> GGTGGGG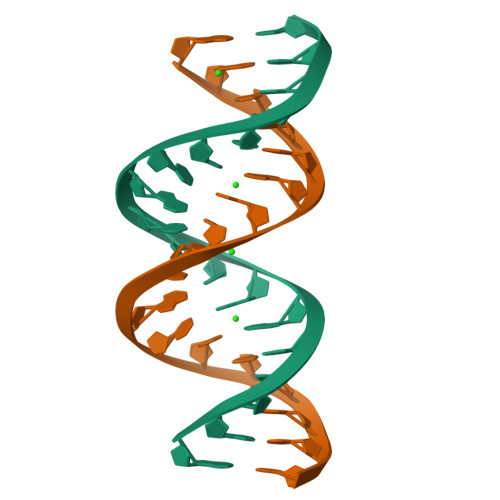CTTGCCCCACC> KRIVACDDPDFLTSYFAHSRLHHLSAWKANLKDKFLNENIHKYTKITDKDTYIIFHIDFDCFFATVAYLCRSSSFSACDFKRDPIVVCHGTKNSDIASCNYVARSYGIKNGMWVSQAEKMLPNGIKLISLPYTFEQFQLKSEAFYSTLKRLNIFNLILPISIDEAVCVRIIPDNIHNTNTLNARLCEEIRQEIFQGTNGCTVSIGCSDSLVLAALALKMAKPNGYNITFKSNLSEEFWSSFKLDDLPGVGHSTLSRLESTFDSPHSLNDLRKRYTLDALKASVGSKLGMKIHLALQGQDDEESLKILYDPKEVLQRKSLSIDINWGIRFKNITQVDLFIERGCQYLLEKLNEINKTTSQIT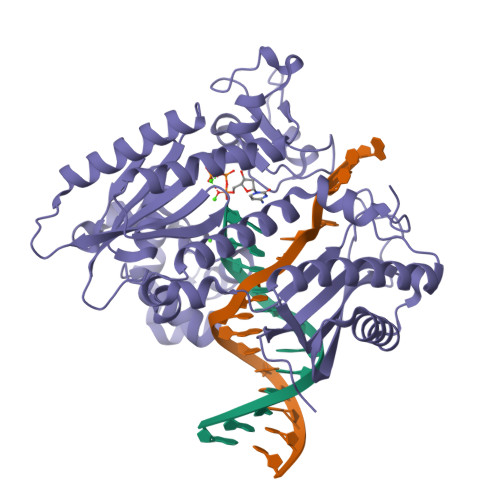LKLMRRCKDAPIEPPKYMGMGRCDSFSRSSRLGIPTNEFGIIATEMKSLYRTLGCPPMELRGLALQFNKLVDVGPDNNQLK>[2x]MAGDTTITIVGNLTADPELRF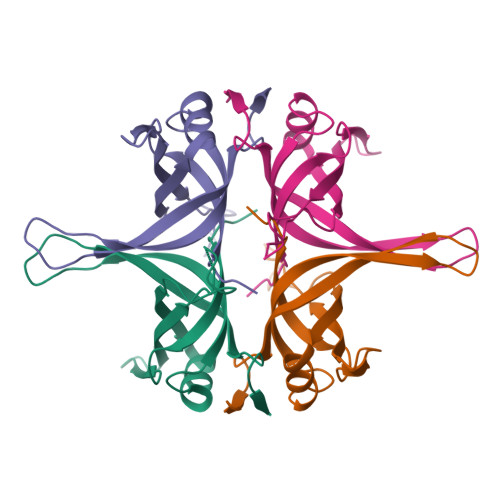TPSGAAVANFTVASTPRIYDRQTGEWKDGEALFLRCNIWREAAENVAESLTRGARVIVSGRLKQRSFETREGEKRTVIEVEVDEIGPSLRYATAKVNKASRSGGFGSGSRPAPAQTSSASGDDPWGSAPASGSFGGGDDEPPF N-{2-[7-(methylsulfamoyl)naphthalen-1-yl]ethyl}acetamide 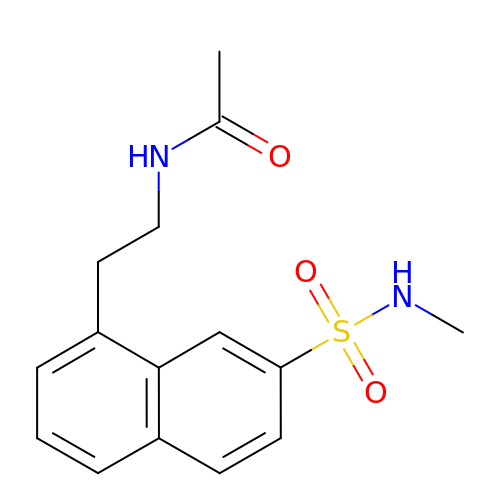| C15 H18 N2 O3 S | LMMCCCKILDSFAH-UHFFFAOYSA-N> PPTLQRCCRQLRNVSPFCRCPSLRQAVQSAQQQQGQVGPQQVGHMYRVASRIPAICNLQPMRCPF;> QRCRHQFQTQQRLRACQRVIQ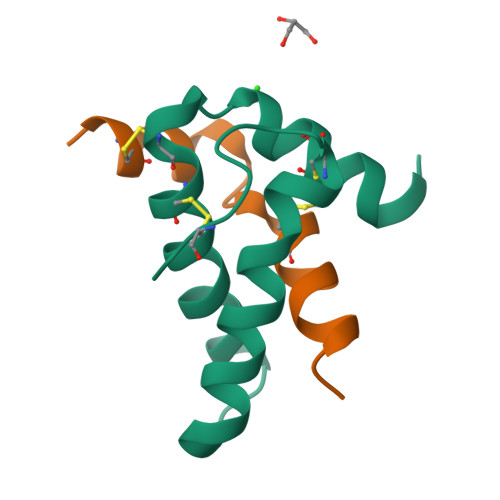RWSQ>SNAMHMLRIAKEALTFDDVLLVPAHSTVLPNTADLRTRLTKNIALNIPMVSASMDTVTEARLAIALAQEGGIGFIHKNMSIEQQAAQVHQVKIFESGGAKDFHKAESKPNACKDEQGRLRVGAAVGAAPGNEERVKALVEAGVDVLLIDSSHGHSEGVLQRIRETRAAYPHLEIIGGNVATAEGARALIEAGVSAVKVGIGPGSICTTRIVTGVGVPQITAIADAAGVANEYGIPVIADGGIRFSGDISKAIAAGASCVMVGSMFAGTEEAPGEVILYQGRSYKAYRGMGSLGAMSKGSSDRYFQTDNAADKLVPEGIEGRIAYKGHLKEIIHQQMGGLRSCMGLTGSATVEDLRTKAQFVRISGAGMKESHVHDVQ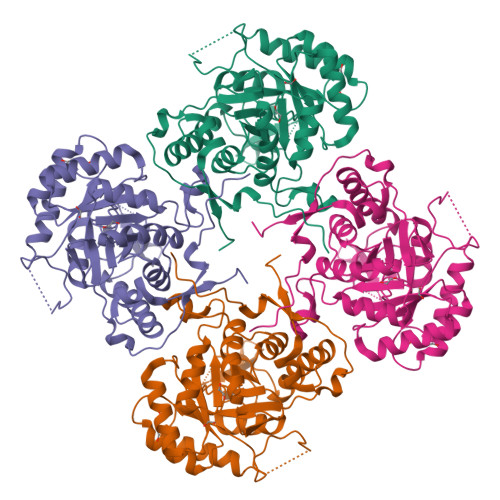ITKEAPNYRLG[2x]> VEDATRSDSTTQMSSTPEVVYSSAVDSKQNRTSDFDANWKFMLSDSVQAQDPAFDDSAWQQVDLPHDYSITQKYSQSNEAESAYLPGGTGWYRKSFTIDRDLAGKRIAINFDGVYMNATVWFNGVKLGTHPYGYSPFSFDLTGNAKFGGENTIVVKVENRLPSSRWYSGSGIYRDVTLTVTDGVHVGNNGVAIKTPSLATQNGGDVTMNLTTKVANDTEAAANITLKQTVFPKGGKTDAAIGTVTTASKSIAAGASADVTSTITAASPKLWSIKNPNLYTVRTEVLNGGKVLDTYDTEYGFRWTGFDATSGFSLNGEKVKLKGVSMHHDQGSLGAVANRRAIERQVEILQKMGVNSIRTTHNPAAKALIDVCNEKGVLVVEEVFDMWNRSKNGNTEDYGKWFGQAIAGDNAVLGGDKDETWAKFDLTSTINRDRNAPSVIMWSLGNEMMEGISGSVSGFPATSAKLVAWTKAADSTRPMTYGDNKIKANWN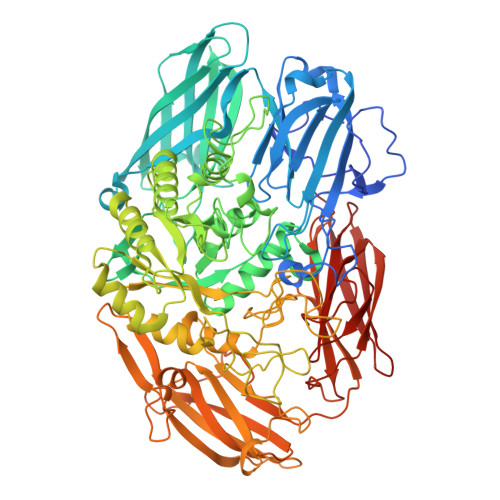ESNTMGDNLTANGGVVGTNYSDGANYDKIRTTHPSWAIYGSETASAINSRGIYNRTTGGAQSSDKQLTSYDNSAVGWGAVASSAWYDVVQRDFVAGTYVWTGFDYLGEPTPWNGTGSGAVGSWPSPKNSYFGIVDTAGFPKDTYYFYQSQWNDDVHTLHILPAWNENVVAKGSGNNVPVVVYTDAAKVKLYFTPKGSTEKRLIGEKSFTKKTTAAGYTYQVYEGSDKDSTAHKNMYLTWNVPWAEGTISAEAYDENNRLIPEGSTEGNASVTTTGKAAKLKADADRKTITADGKDLSYIEVDVTDANGHIVPDAANRVTFDVKGAGKLVGVDNGSSPDHDSYQADNRKAFSGKVLAIVQSTKEAGEITVTAKADGLQSSTVKIATTAVPGTSTE The T4 bacteriophage gp41 helicase and gp61 primase assemble into a primosome to couple DNA unwinding with RNA primer synthesis for DNA replication. The domain architecture of the gp41 helicase resembles the bacterial DnaB helicase13,14 with an NTD and a RecA-like CTD that are connected by a linking helix (LH). The gp61 primase is composed of an N-terminal ZBD and a C-terminal RPD that are linked by an 18-residue flexible loop. Here we report a series of cryo-EM structures of T4 primosome assembly intermediates.

We hypothesized that the absence of the RNA primer density in our primosome EM map was due to slow ATPγS hydrolysis by the WT gp41 helicase. Therefore, we utilized an inactive gp41 helicase mutant with an E227Q substitution in the walker-B motif that abolished the ATP-hydrolysis activity, and assembled a T4 primosome with the WT gp61 primase and the ssDNA/RNA primer substrate. The gp61 primase region achieved ~4.0 Å local resolution where the pentaribonucleotide primer was observed to form a short hybrid duplex with the template DNA that was absent in the WT primosome map. Interestingly, we found that the gp61 RPD rotated around the HIM2 by ~6° away from the ZBD to engage the ssDNA/RNA duplex, as compared to the gp61 primase in the WT primosome where the RNA primer is missing. Superposition of the gp61 primase structures of the WT and mutant primosomes shows that the RPD moves outward by 4 Å to accommodate the ssDNA/RNA duplex in the mutant structure. In the mutant primosome, rotation of the gp61 RPD caused the ssDNA template to rotate and interact more extensively with the gp61 ZBD as compared to the ssDNA in the WT primosome. Interestingly, the 3′-OH of the primer has passed over the catalytic site in the mutant structure, such that no additional ribonucleotides can be added in this configuration. This is consistent with the predominant 5-nt length of primers synthesized by the gp61 primase. We therefore assigned the mutant T4 primosome structure as in a post-primer-synthesis state. Indeed, we found that the linker loop stretched and became ordered in the mutant T4 primosome bound to a completed 5-nt RNA primer, as compared to the disordered linker loop in the ssDNA template-bound WT primosome.

>[6x]MVEIILSHLIFDQAYFSKVWPYMDSEYFESGPAKNTFKLIKSHVNEYHSVPSINALNVALENSSFTETEYSGVKTLISKLADSPEDHSWLVKETEKYVQQRAMFNATSKIIEIQTNAELPPEKRNKKMPDVGAIPDIMRQALSISFDSYVGHDWMDDYEARWLSYMNKARKVPFKLRILNKITKGGAETGTLNVLMAGVNVGKSLGLCSLAADYLQLGHNVLYISMQMAEEVCAKRIDANMLDVSLDDIDDGHISYAEYKGKMEKWREKSTLGRLIVKQYPTGGADANTFRSLLNELKLKKNFVPTIIIVDYLGICKSCRIRVYSENSYTTVKAIAEELRALAVETETVLWTAAQVGKQAWDSSDVNMSDIAESAGLPATADFMLAVIETEELAAAEQQLIKQIKSRYGDKNKWNKFLMGVQKGNQKWVEIE;> SIPWIDNEFAYRALAHLPKFTQVNNSSTFKLRFRCPVCGDSKTDQNKARGWYYGDNNEGNIHCYNCNYHAPIGIYLKEFEPDLYREYIFEIRKEKGKSRPIEKPKELPKQPEKKIIKSLPSCVRLDKLAEDHPIIKYVKARCIPKDKWKYLWFTTEWPKLVNSIAPGTYKKEISEPRLVIPIYNANGKAESFQGRALKKDAPQKYITIEAYPEATKIYGVERVKDGDVYVLEGPIDSLFIENGIAITGGQLDLEVVPFKDRRVWVLDNEPRHPDTIKRMTKLVDAGERVMFWDKSPWKSKDVNDMIRKEGATPEQIMEYMKNNIAQGLMAKMRLSKYAK> MKFLFYLSADNLEIARKEVLVLAERYGWVEDYQFEERLLLLDYAGEKFFERLAYTNEVTKIYDICSVSELEQVFSEIPVYDRLCCVRVKGGKGKTALERKLGALLWKRGAKVSVSNPEIVYKVYIQDDKCYVGLLEFERDTRQFFLRRPDRRPFLMPSAIKPKLARALVNLTGVLEGETLLDPMCGTGSFLIEAGLMGINPIGIDFIEKIVRGCRVNLEYYGIEGSVLLGDAKNLPLRDESVRGIATDYPYLRSTKAAGTLDELYSKTSEEFERVLKKGGRAAIVTNIDVESFFSNFEIEMKTEER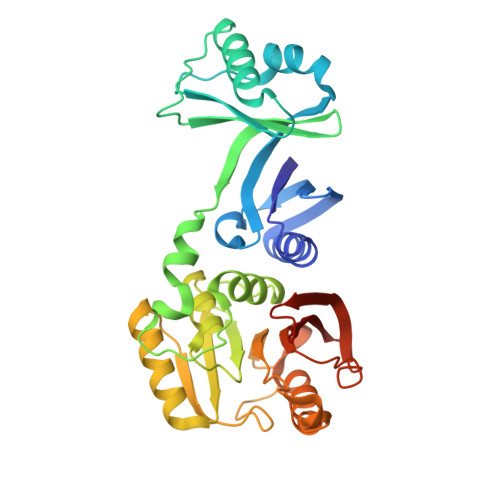VHGSLTRRIYLLRRHHHHHH4-(METHYLSULFONYL)BENZENECARBOXIMIDAMIDE | C8 H10 N2 O2 S | 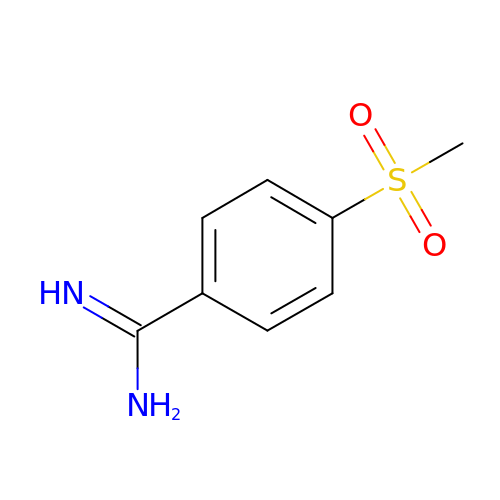ANPBNAUKOUYEGJ-UHFFFAOYSA-N> MLKQVEIFTDGSCLGNPGPGGYGAILRYRGREKTFSAGYTRTTNNRMELMAAIVALEALKEHCEVILSTNSQ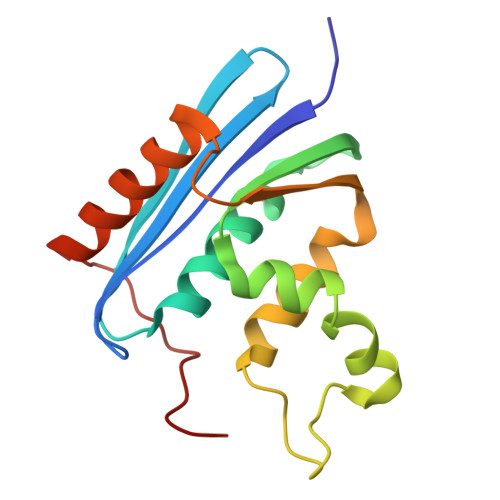YVRQGITQWIHNWKKRGWKTADKKPVKNVDLWQRLDAALGQHQIKWEWVKGHAGHPENERCDELARAAAMNPTLEDTGYQVEV>GDYT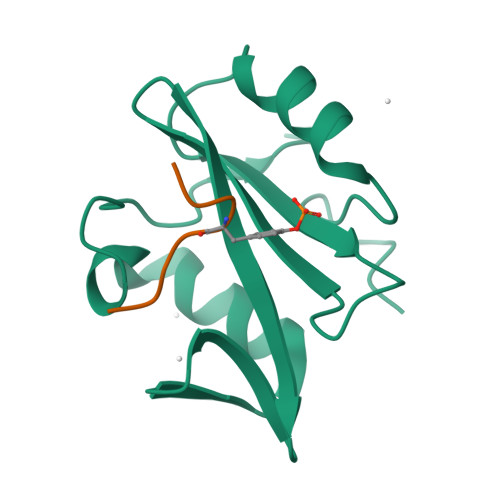AYPWFAGNMERQQTDNLLKSHASGTYLIRERPAEAERFAISIKFNDEVKHIKVVEKDNWIHITEAKKFDSLLELVEYYQCHSLKESFKQLDTTLKYPYKSRERSASRASSRSP[3x];>XTPEAPPCYMDVIX[3x]> MTEAVAFPQNRSCPYHPPTAYEPLREERPLSRVTLWNGRQVWFVTGHQAARALLGDQRLSTDSTREDFPLPTERSESLRRQRRGALLGWDDPEHNEQRRMLIPSFTLRRAESMRPRIQAIVDRLLDDMIAAGPSAELVGAFALPVPSMVICELLGVPYGDHEFFEEQSRRLLRGPAAEDIEKAFRSLEGYFGELIETKRTDPGEGVIDDLVARQREEGRPDDDELVQFATVLLVAGHETTANMISLATYTLLEHPAR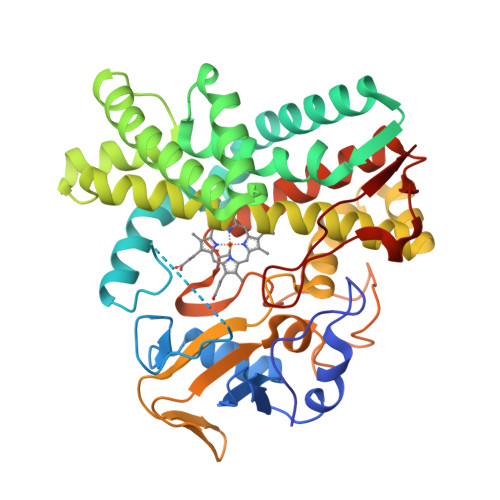LAELRADPGLVPAAVEELLRFLSIADGLVRVAREDVPVGDQVIRAGEGVVFPTSLINRDDSVYEHPDTLDWSRSARHHVAFGFGIHQCLGQNLARIELEIALGTLLRRLPGLRLAAPADRIPFKPGDTIQGMLELPVTW>MGSCCSCLKDSSDEASVSYLEDKDQLDFYSGGPLKALTTLVYSDNLNLQRSAALAFAEITEKYVRQVSREVLEPILILLQSQDPQIQVAACA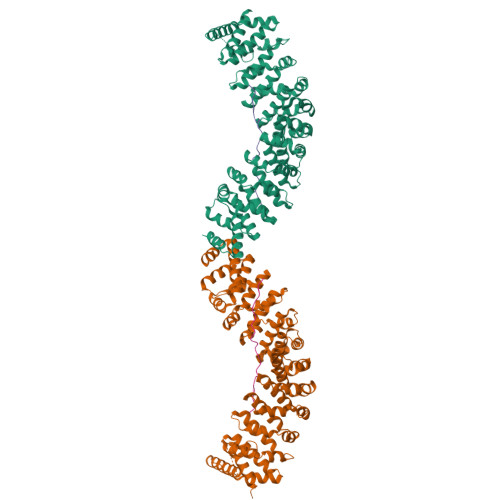ALGNLAVNNENKLLIVEMGGLEPLINQMMGDNVEVQCNAVGCITNLATRDDNKHKIATSGALIPLTKLAKSKHIRVQRNATGALLNMTHSEENRKELVNAGAVPVLVSLLSSTDPDVQYYCTTALSNIAVDEANRKKLAQTEPRLVSKLVSLMDSPSSRVKCQATLALRNLASDTSYQLEIVRAGGLPHLVKLIQSDSIPLVLASVACIRNISIHPLNEGLIVDAGFLKPLVRLLDYKDSEEIQCHAVSTLRNLAASSEKNRKEFFESGAVEKCKELALDSPVSVQSEISACFAILALADVSKLDLLEANILDALIPMTFSQNQEVSGNAAAALANLCSRVNNYTKIIEAWDRPNEGIRGFLIRFLKSDYATFEHIALWTILQLLESHNDKVEDLVKNDDDIINGVRKMADVTFERLQRSGIDVKNPGSNNNPSSNDNNSNNNDTGSEHQPVEDASLELYNITQQILQFLH[2x];>[2x]GGNSSTSALNSRRNSLDKSSNKQGMSGLPPIFGGESTSYHHDNKIQKYNQLGVEEDDDDENDRLLNQMGNSATKFKSSISPRSIDSISSSFIKSRIPIRQPYHYSQPTTAPFQAQAKFHKPANKLIDNG> GPGTQEETNFKSLVHDLFQKVEEAKSSLAMNRSRGKVLDAIIQEKKS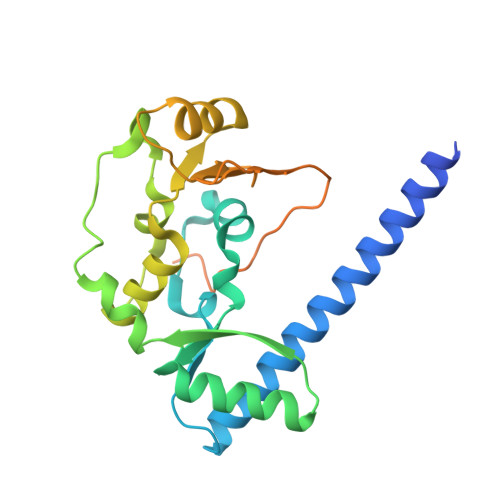GRIPGIYGRLGDLGAIDEKYDVAISSCCHALDYIVVDSIDIAQECVNFLKRQNIGVATFIGLDKMAVWAKKMTEIQTPENTPRLFDLVKVKDEKIRQAFYFALRDTLVADNLDQATRVAYQKDRRWRVVTLQGQIIEQSGTMTGGGSKVMKGRMGSSLVIEISEEEVNKMESQLQNDSKKAMQIQEQKVQLEERVVKLRH>MGSSHHHHHHSSGAIIPPWIHVPDHSRFFVIKSSSLEHVKKSFYNGIWSSTFYGNKRLSEAYESLPQGAKIYLLFSVNASGRFCGVAEMSSNLREDLDTSIWGDNSRYRHAFKVRWIVVRDVHNRSLKQFLIPANDMKPVTNSR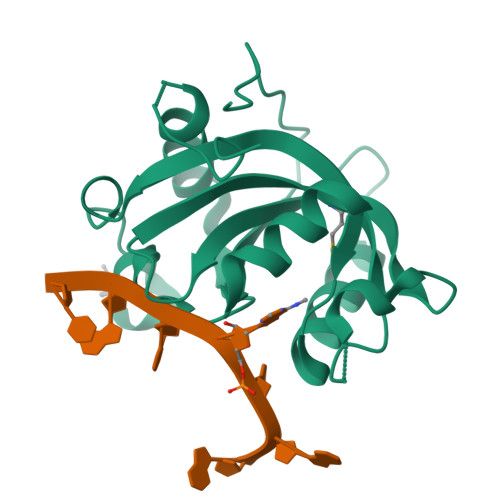DTQEIPATISKSILKLFKYEQSEVQSFLDDDYS[6x]Acid sphingomyelinase (ASMase, ASM, SMPD1) is an enzyme found in lysosomes and in the extracellular space where it catalyses the conversion of sphingomyelin, a major component of membranes, into ceramide and phosphocholine. ASMase consists of an N-terminal saposin domain and a C-terminal catalytic domain. To gain insight into the molecular mechanism of ASMase function and the interplay between its domains, we determined crystal structures of the full-length protein from mouse that reveal a conformational flexibility of the saposin domain. In one conformation, the saposin domain adopts a globular closed form independent of the catalytic domain, while in the other conformation, it assumes an open V-shaped fold that establishes an extended interface with the catalytic domain.

As observed with other saposins, ASMasesap adopts either a closed or open conformation depending on environmental conditions. By contrast, the open form of ASMasesap assumes a V-shaped conformation with its hydrophobic core exposed and its position shifted on ASMasecat such that one face of helix α3 forms an extensive 1,318 Å2, hydrophobic interface with ASMasecat. The interface presumably stabilizes the open conformation of ASMasesap, allowing it to dock onto membrane surfaces, and possibly deliver lipids to the active site. The location on open ASMasesap responsible for membrane lipid docking under physiological conditions likely includes its hydrophobic surface, which in the crystal is buried by a symmetry-related saposin domain reminiscent of the ‘handshake' clasp observed in saposin B dimers. Indeed, crystallization in the presence of lipids rearranges the saposin dimer and reveals lipid molecules bound within it. In addition, the top edge of helix α2, which is lined with a ridge of positively charged residues, is appropriate for interaction with anionic intra-lysosomal vesicles. In the presence of anionic membranes, open ASMasesap becomes prevalent, docks onto the membrane surface and concomitantly forms an interface with the catalytic domain activating it for sphingomyelin hydrolysis.

>DRHHHHHHKLNLTCPACKVLFTALNHGLKKEPNVARVGSVAIKICKMLNIAPLDVCQSAVHLFEDDVVEVWTRSVLSPSEACGLLLGSSCGHWDIFSTWNISLPSVPKPPPKPPSPPAPGAPVSRVLFLTDLHWDHEYLEGTDPYCADPLCCRRGSGWPPNSQKGAGFWGEYSKCDLPLRTLESLLKGLGPAGPFEMVYWTGDIPAHDVWQQSRQDQLRALTTITDLVRKFLGPVPVYPAVGNHESTPVNGFPPPFIKGNQSSQWLYEAMAKAWEPWLPADALHTLRIGGFYALTPRPGLRLISLNMNFCSRENFWLLINSTDPAGQLQWLVEELQAAENRGDKVHIIGHIPPGHCLKSWSWNYYKIIARYENTLAGQFFGHTHVDEFEIFYDEETLSRPLAVAFLAPSATTFINLNPGYRVYQIDGNYPGSSHVVLDHETYILNLTQANAAGGTPSWKRLYRARETYGLPDAMPASWHNLVYRMRDDEQLFQTFWFLYHKGHPPSEPCGTPCRLATLCAQLSARADSPALCRHLMPN[4x]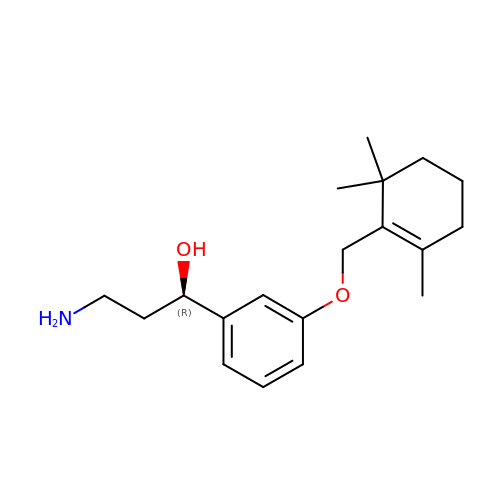(1R)-3-amino-1-{3-[(2,6,6-trimethylcyclohex-1-en-1-yl)methoxy]phenyl}propan-1-ol | C19 H29 N O2 | IMAIQFBFQHDLHJ-GOSISDBHSA-N>GHMTLYRLHEADLEIPDAWQDQSINIFKLPASGPAREASFVISRDASQGDAPFADYVARQLENAEKQLPGFKLHKRWDINIHGHAAVLLDYQWQREGRD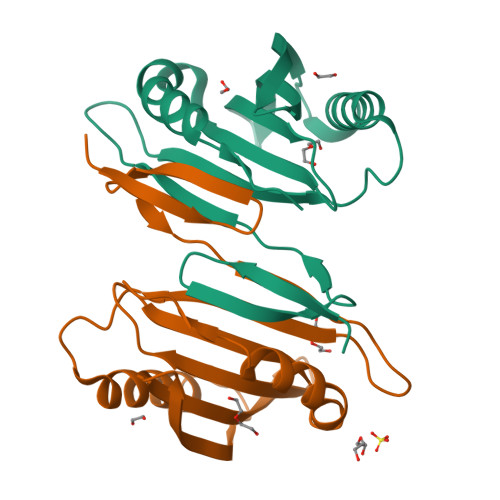LMLRQVFIERRPAVLITTLTTTPADLPHHEPAWKQAMQTLVPRPTPSGS[2x]>[2x]GAMDGSAQSSERRVVAHMPGDIIIGALFSVHHQPTVDKVHERKCGAVREQYGIQRVEAMLHTLERINSDPTLL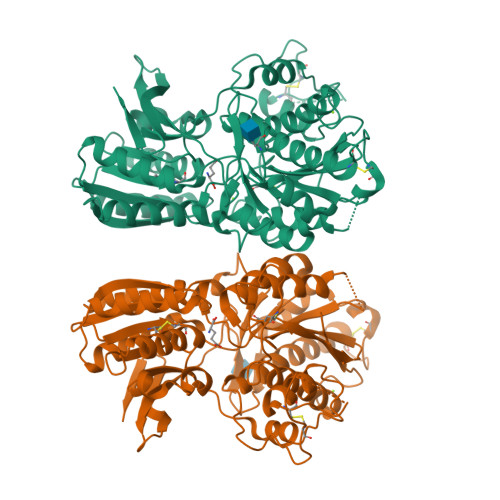PNITLGCEIRDSCWHSAVALEQSIEFIRDSLISSEEEEGLVRCVDGSSSSFRSKKPIVGVIGPGSSSVAIQVQNLLQLFNIPQIAYSATSMDLSDKTLFKYFMRVVPSDAQQARAMVDIVKRYNWTYVSAVHTEGNYGESGMEAFKDMSAKEGISIAHSYKIYSNAGEQSFDKLLKKLTSHLPKARVVACFCEGMTVRGLLMAMRRLGLAGEFLLLGSDGWADRYDVTDGYQREAVGGITIKLQSPDVKWFDDYYLKLRPETNHRNPWFQEFWQHRFQCRLEGFPQENSKYNKTCNSSLTLKTHHVQDSKMGFVINAIYSMAYGLHNMQMSLCPGYAGLCDAMKPIDGRKLLESLMKTNFTGVSGDTILFDENGDSPGRYEIMNFKEMGKDYFDYINVGSWDNGELKMDDDEVWSKKSN> SDHFLVINGKNCCVFRDENIAKVLPPVLGLEFVFGLLGNGLALWIFCFHLKSWKSSRIFLFNLAVADFLLIICLPFLTDNYVHNWDWRFGGIPCRVMLFMLAMNKQGSIIFLTVVAVARYFRVVHPHHFLNKISNRTAAIISCFLWGLTIGLTVHLLYTNMMT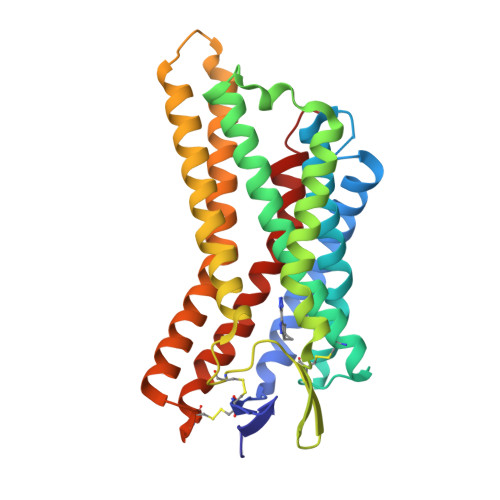KNGEAYLCSSFSICYNFRWHDAMFLLEFFLPLAIILFCSGRIIWSLRQRQMDRHAKIKRAINFIMVVAIVFIICFLPSVAVRIRIFWLLYKYNVRNCDIYSSVDLAFFTTLSFTYMNSMLDPVVYYFSSPS>[2x]DNVVRKDVSHLTVDEVQALHGALHDVTASTGPLSFEDITSYHAAPASCDYKGRKIACCVHGMPSFPFWHRAYVVQAERALLSQRKTVGMPYWDWTETLTQLPALVTEPIFIDSLGGKTQPNYWHRGEIAFANKATARAVDDRLFEKVETGHYTKLMESVLDALERDEFCKFEIQFELAHNAIHYLVGGKYEYSMSNLDYTAYDPIFFLHHSNVDRIFAIWQRLQELRGKNPKAIDCAHELARQELEPFNRDTNPVPITKQHSRPVDLFDYHQLGYSYDSLNLNGMTPEELKIKLDERHSKERAFASFRLKGFGGSANVVVYACLPDSDPRSDDHCEKAGDFFVLGGSTEAPWVFYRPYFFDVTKAVQRLGVALSGHYYVKTELFSVNGTSLSPDILPQPTVAYRPGKGHIDPPVHHRQNEDYIVRKNIDHLTRSETYELRKAMERFQADTSVDGFQATVEYHGLPARCPEPDAKVRFACCMHGMASFPHWHRLFVTQVEDALVRRGPPIGVPYWDWTKPMTHLPDLAASEDYVDPNGHTRHNPFFNANISFEEEHHHTSRSIDARLFAPAAYGDHTALFDGILYAFEQEDFCDFEIQFELVHNSIHAWIGGSEDYSMSTLHYAAFDPIFYLHHSNVDRLWAIWQALQIRRQKPYRAHCAQSIEQLPMKPFAFPSPLNNNEKTHSNSVPTDIYDYEETLHYSYDDLTFGGMNLDEIEETIHHRQQHERVFAGSLFGGIGKSALVNIFINKPGSSPHKAGDIAILGGTKEMPWAFDRLYKVEITDALKALALDVDGDYEVTFDIHDMHGNKLSSDLIPHPAVISEPAHPSFEDVTTSLRIRKNVDYLTPEETNDLRHALDLLEKDPSAGGFDQLGAFHGEPKWCPNPEAEHKVACCVHGMAVFPHWHRLLALQAENALRRHGYSGAFPYWDWTHPISKLPDLVTPETYTDPSDNQDKHNPWYNGHIETVDQDTTRNVRGDLYQQPEFGHSTDIAPQVLLALEQDDFCSFEVQYEISHNFIHALVGGTTPYGMASLRYTAYDPIFFLHHSNTDRIWAIWQALQKYRGKPYNTANCAIASMRKPLQPFGLSSDVNPDIITREHAIPFDVFNYRGNFHYKYDTLEFNGLSISQLNRELDKIKSHDRVFAGFLLSGIKKSVLVKFNVCAPPHDCHPAGEFYLLGDENEMAWAYDRVFKYDTTNVLDENNLHFYDHIFITYEVFDLHGTSLGTDIFHKANVIHDSGTGSREHDRYVEEVTGASHIRKNLNDLNLGEMESLRAAFLHIQNDGTYESIAQYHGKPGKCELNHRSIACCVRGMPTFPQWHRLYVAQVENALLKMGSSVAVPYWEWTAPIDHLPGLIDDATYFNSRQQRYDPNPFFRGKISFENAVTTRDPQEELFNSEYMQNNVLLALEQDNYCDFEIQFELVHNALHSLLGGKGQYSMSSLDYSAFDPVFFLHHANTDRLWAIWQELQRYRGLPYEEANCAINLMHQPLMPFSDPNENHGNVTLKHSKPQDCFDYRNNFGYKYDNLEFHHLSIPSLDATLKARKEHDRVFAGFLLHNIGTSADISIYICLPDGSGGNDCSHKAGTFYVLGGETEMPFVFDRLYKFEITEALHKLGVKLHGGLFDLELDIVAYNGSHLDSHIFDPTIIFEPGIDTHVLDHDNTEEILVRKNIIDLSPRERVSLVKALKGMQNDRSADGYQAIASFHALPPLCPNPSAANRFACCVHGMATFPQWHRLYTVQFQDALRRHGSLVGIPYWDWTKPVSELPKLLSAETFHDPIHNVNVSNPFFKADIEFEGDGVHTERDIQPDFLFHSGDHEGYHNWFFETVLLALE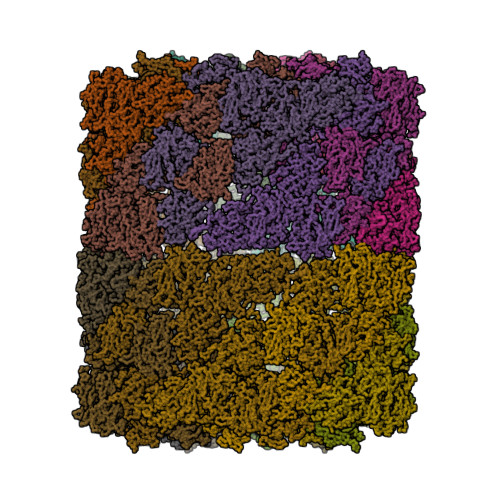QEDYCDFEIQFEIAHNGIHTWIGGSAKYGMGHLHYASYDPIFYIRHSQTDRIWAIWQELQKYRGLSGSEANCAIELMRTPLKPFSFGAPYNLNSHTQEFSKPEDTFDYKKFGYRYDNLELEGRSVAHIDELIKERQEHDGTFAGFLLKGFGTSATVTLKICRDDYTCENAGYFTVLGGSAEMPWAFDRLYKYDITKTLDHMNLRHEDTFYINGTVTAYDGTVLPGDLIPPASIIFVPGRHNLNSRKHTPNKIRHELTSLSSRDVASLKAALTSLQKDDGPNGYQAIAAFHGLPAQCHDTSGHQIACCIHGMATFPHWHRLYTLQLEWALAKHGSSVAVPYWDWTRPITELPHILTDGEYYDFWQDAVMPNPFSRGHVKFENTFTVRNVRKALFKLSPIGKHSVLFDQALLALEQTDYCDFEVQFEVMHNTIHYLIGGRQTYAFSSLHYASYDPIFFIHHSFVDKIWAIWEELQSRRHLQFNGADCAVSLMSKAMRPFNKDFNHNPFTKKHAVPNTLFDYEDLGYNYDNLEISGLNLKEIEALIAKRKSHARVFAGFLLFGIGTSADIHLDICKTSDGCHHAGVLFILGGSAEMHWAYNRLYKYDITEALHEFGINPEDVFHADEAFFLKVSVVAVDGTVLPPSLLHEPTILYEPGVGHHEDHESGSLAGSGVRKDVNTLTTAETENLRKALRGVKEDHGYNGFQAIAAFHGKPAMCPMADGHNLSCCTHGMATFPHWHRLYTKQMEGALKAHGSHVGLPYWDWTAAFSHLPTLVTDNDNNPFHDGTIEYLNVTTTRSPRDLLFNDPEHGSESFFYRQVLFALEQTDFCKLEVQFEITHNAIHSWTGGHSPYGMSTLDFTAYDPLFWLHHSNTDRIWAIWQALQKYRGLPYNHANCEIQAMKTPLRPFSDNINHNPVTKANSRPVDVFEYNRLRYQYDNLVFHGHTIPELDHMLEERKKHDRIFAAFLLSGIKKSADVVFEICEPNHECVFAGTFAILGGELEMPWSFDRLFRYDITKVMQQQHLRHDSDFSFKVKVVGTDDIELPPGILKEPTIEFEPALGDGLKHEDEGHDDRLSHVLIRKEVDLLSLKEANAIKDALYKLQNDHSKGGFEEIAGYHGYPNKCPEKGDDKYPCCVHGMPIFPHWRRLHTIQMERALKNHGSQIGIPYWNWTKRMSSIPAFFGDDSNNNPFYKYHIRAVNQYTTRDVDVELFNQTKFGEYDYLYYSTLQVLEENSFCGFEVQYEILHSAVHAWLGGAGKYSMSTLEYSAYDPVFMIHHSSLDRIWILWQQLQKRRMKLYYAADCAGDLMKFPMHPFSYKSENEDEFTRVNSVPNIVFDHYKFNYDYDNMRIRGHDINELEAIINELRNKDRIFAGFVLSGIRITATVKVFIHGTGATDHEEFAGKFAILGGEKEMPWAYERLLKLDITDAVHHLHLKDEEIRFRMEVTAYNGVPVSTKLADPLIAHRPA> TSSANEDMPVEKILEAELAVEPKTETYVEANMGLNPSSPNDPVTNICQAADKQLFTLVEWAKRIPHFSELPLDDQVILLRAGWNELLIASFSHRSIAVKDGILLATGLHVHRNSAHSAGVGAIFDRVLTELVSKMRDMQMDKTELGCLRAIVLFNPDSKGLSNPAEVEALREKVYASLEAYCKHKYPEQPGRFAKLLLRLPALRSIGLKCLEHLFFFKLIGDTPIDTFLMEMLEAPHQAT;> MSKESVRNDRNKKKKEVPKPECSESYTLTPEVGELIEKVRKAHQETFPALCQLGKYTTNNSSEQRVSLDIDLWDKFSELSTKCIIKTVEFAKQLPGFTTLTIADQITLLKAACLDILILRICTRYTPEQDTMTFSDGLTLNRTQMHNAGFGPLTDLVFAFANQLLPLEMDDAETGLLSAICLICGDRQDLEQPDRVDMLQEPLLEALKVYVRKRRPSRPHMFPKMLMKITDLRSISAKGAERVITLKMEIPGSM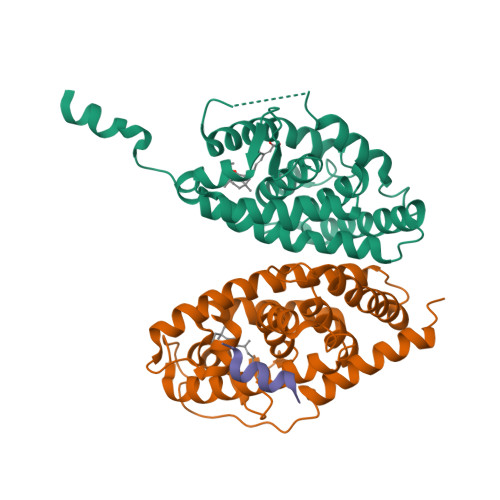PPLIQEMLENSEGLD;> KHKILHRLLQDSS>[2x]GSSLISKTIKYDPAKDKLITLACGCFWGTEHMY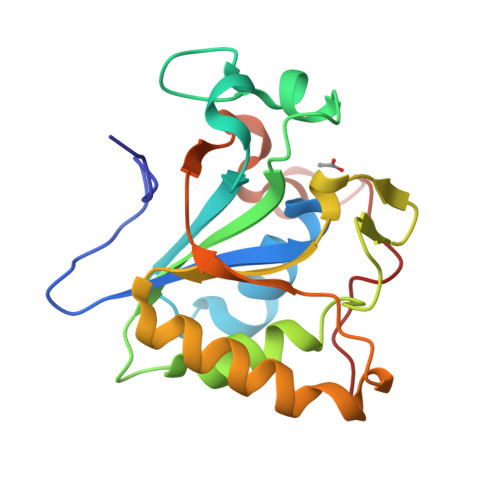RKYLNDRIVDCKVGYANGEESKKDSPSSVSYKRVCGGDTDFAEVLQVSYNPKVITLRELTDFFFRIHDPTTSNSQGPDKGTQYRSGLFAHSDADLKELAKIKEEWQPKWGNKIATVIEPIKNFYDAEEYHQLYLDKNPQGYACPTHYLREM> MTAKTIRHYLQFKDFSLEDYEYVLERTGILKRKFKNYETYHPLHDRTLAM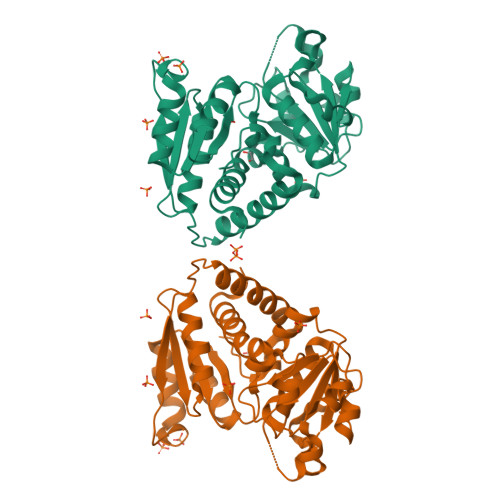IFEKSSTRTRLSFEAGIFQLGGHAVFMSTRDTQLGRGEPVEDSAQVISRMVDIIMIRTFEQDIIQRFAENSRVPVINGLTNEYHPCQVLADIFTYYEHRGPIRGKTVAWVGDANNMLYTWIQAARILDFKLQLSTPPGYALDAKLVDAESAPFYQVFDDPNEACKGADLVTTDVWTSMGFEAENEARKRAFADWCVDEEMMSHANSDALFMHCLPAHRGEEVTAGVIDGPQSVVWDEAENRLHVQKALMEFLLLGRLNH> GSHMSNTQTVLPFTGLNTPSGVAVDSAGTVYVTDHGN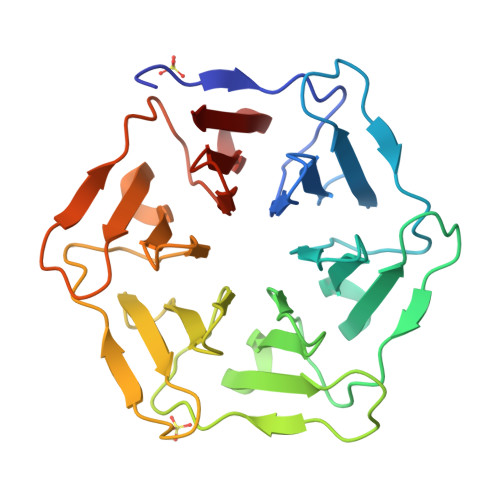NRVVKLAAGSNTQTVLPFTGLNTPSGVAVDSAGTVYVTDHGNNRVVKLAAGSNTQTVLPFTGLNTPSGVAVDSAGTVYVTDHGNNRVVKLAAGSNTQTVLPFTGLNTPSGVAVDSAGTVYVTDHGNNRVVKLAAGSNTQTVLPFTGLNTPSGVAVDSAGTVYVTDHGNNRVVKLAAGSNTQTVLPFTGLNTPSGVAVDSAGTVYVTDHGNNRVVKLAAG> PYVPVHF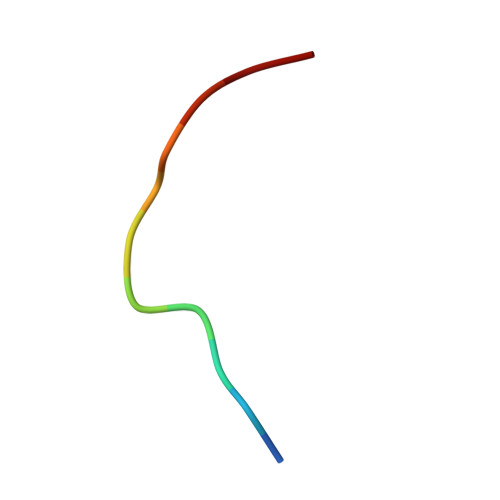NASV N,2,5-trimethyl-3-thiophenesulfonamide | C7 H11 N O2 S2 | 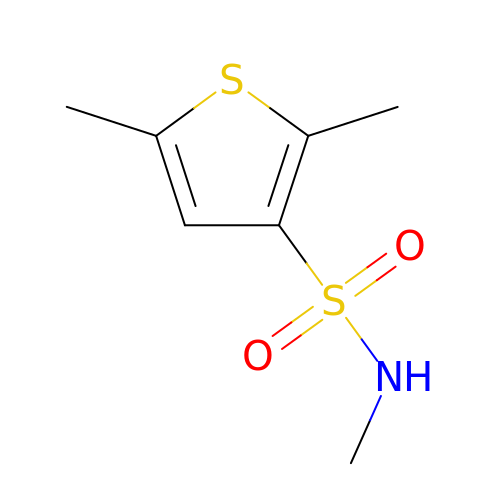MQZNMDAQVFXGMG-UHFFFAOYSA-N> GPHMPGSRQIQLWHFILELL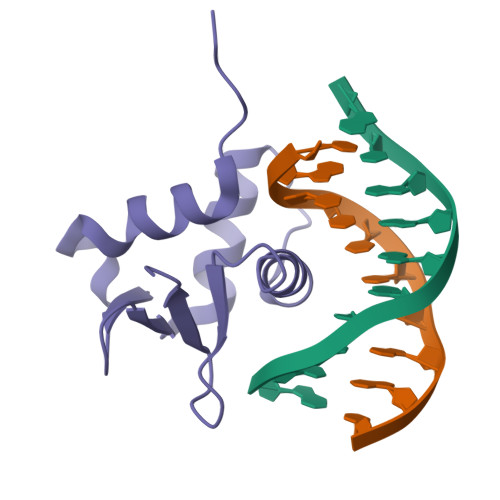RKEEYQGVIAWQGDYGEFVIKDPDEVARLWGVRKCKPQMNYDKLSRALRYYYNKRILHKTKGKRFTYKFNFNKLVLVNYPFIDVGLAGGAVPQSAPPVPSGGS> MAKRPTETERCIESLIAIFQKHAGRDGNNTKISKTEFLIFMNTELAAFTQNQKDPGVLDRMMKKLDLDSDGQLDFQEFLNLIGGLAIACHDSFIKSTQK;> XAMV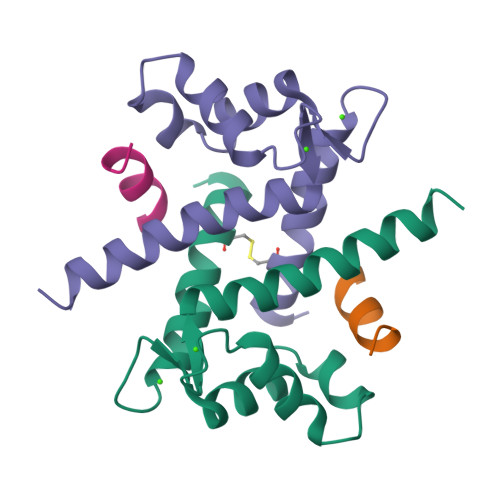SAFLKQAW>MAMTVTEVDLPPIYCPLESAIHPRVHEVEKRAVEWIRRSGMCASEEERAWVIATHSADFFARFAPTAADEDRLLATSLWVYWGFAFDDARCD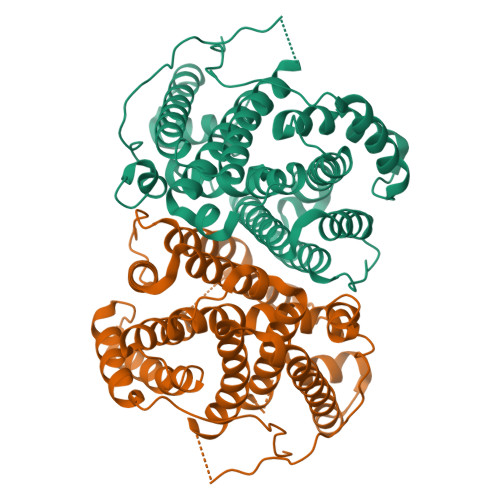NGPLSTRPAQFNALAGRVQRALEAPSAEDNGDRFVPALQDIARRFRSFGTPTQVRRFVHAHRAWLSGVAWQIGNQARGHMPGLDDYLAMRLLSAGGEPTFAMLEIATGAEVPDREMHRPAVRALTEMAIMVAALDNDRHSLRKELSRGHTDQNIYSVLMHHRGMSLQEAVEEATKLRDRILLRFLELHDRVRPGAGAELSTYLQGLRHGIRGNAEWGLRVPRYLSLGRVPDPMEDAPLTWAESPSDSSPSPLPGAPSIAWWWDDALLGA[2x]> SNAMYDTLIIGSGPAGMTAALYAARSNLSVAIIEQGAPGGQMNNTFDIENYPGYDHISGPELAMKMYEPLEKFNVENIYGIVQKIENFGDYKCVLTEDASYEAKTVIIATGAKYRVLGVPGEEYYTSRGVSYCAVCDGAFFRDQDLLVVGGGDSAVEEAIYLTQFAKKVTVVHRRDQLRAQKILQDRAFANDKVDFIWDSVVKEIQGNDIKVSNVLIENVKTGQVTDHAFGGVFIYVGMNPVTGMVKDLEITDSEGWIITDDHMRTSIPGIFAIGDVRQKDLRQITTAVGDGAI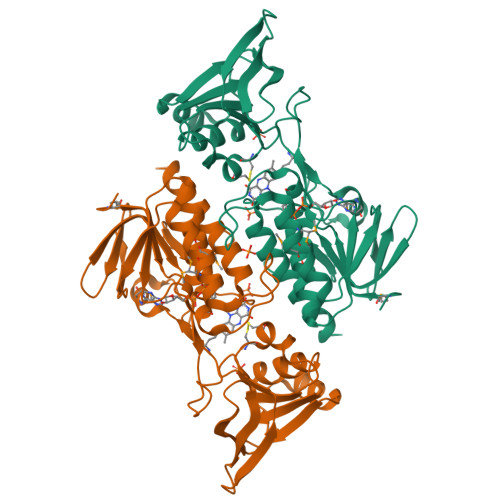AGQGVYHYLESFSS>[3x]MANCERTFIAIKPDGVQRGLVGEIIKRFEQKGFRLVGLKFMQASEDLLKEHYV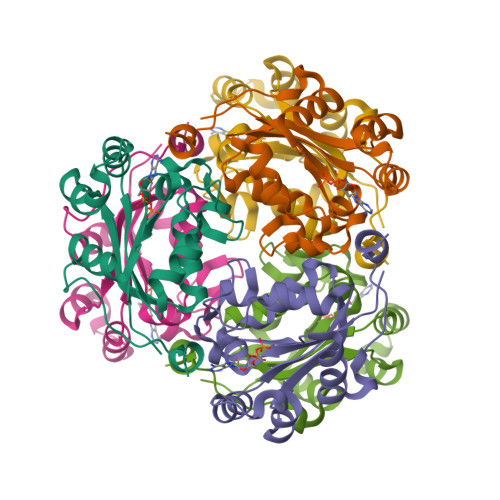DLKDRPFFAGLVKYMHSGPVVAMVWEGLNVVKTGRVMLGETNPADSKPGTIRGDFCIQVGRNIIHGSDSVESAEKEIGLWFHPEELVDYTSCAQNWIYE> STAREQPIFSTRAHVFQIDPATKRNWIPAGKHALTVSYFYDATRNVYRIISIGGAKAIINSTVTPNMTFTKTSQKFGQWADSRANTVYGLGFAS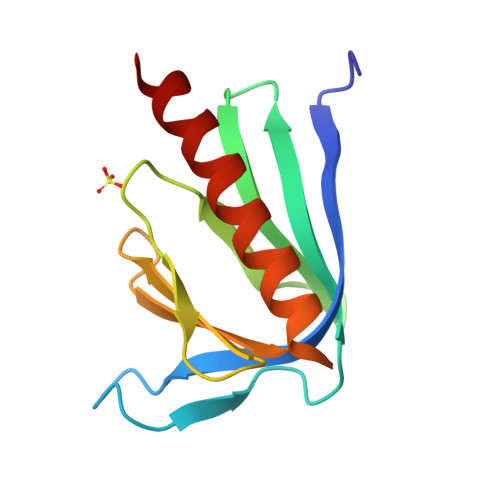EQHLTQFAEKFQEVKEAARLARE>SNAM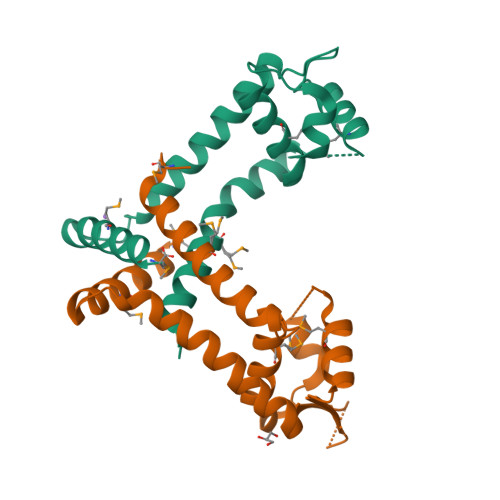KESNHLMDTPYSYLIRSIGMKLKTSADARLAELGLNSQQGRMIGYIYENQESGIIQKDLAQFFGRRGASITSMLQGLEKKGYIERRIPENNARQKNIYVLPKGAALVEEFNNIFLEVEESITKGLTKDEQKQLMSILIKVNRSM[3x]5-[(2S,3R,4S,5R)-5-(hydroxymethyl)-3,4-bis(oxidanyl)oxolan-2-yl]-1-methyl-pyrimidine-2,4-dione | C10 H14 N2 O6 | 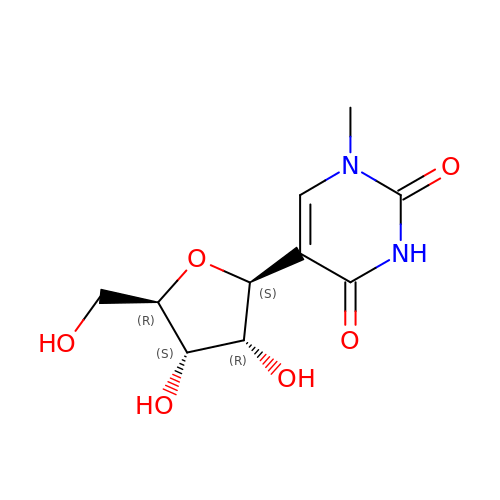UVBYMVOUBXYSFV-XUTVFYLZSA-N>[2x]MTKPLIKPDVDLTDGNFYASRQAREAYRWMRANQPVFRDRNGLAAASTYQAVIDAERQPELFSNAGGIRPDQDALPMMIDMDDPAHLLRRKLVNAGFTRKRVKDKERSIAQLCDTLIDAVCERGECDFVRDLAAPLPMAVIGDM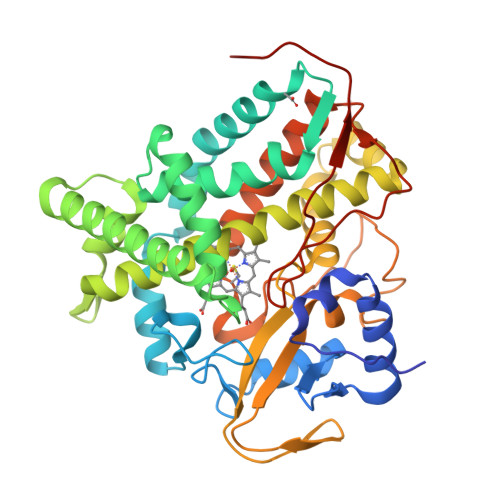LGVLPEQREMFLRWSDDLVTFLSSHVSQEDFQVTIDAFAAYNDFTRATIAARRAEPTDDLVSVLVSSEVDGERLSDDELVMETLLILIGGDETTRHTLSGGSEQLLRNRDQWDLLQSDRELLPGAIEEMLRWTAPVKNMCRMLTADTEFHGTALSEGEKIMLLFESANFDEAVFTDPEKFDIQRNPNSHLAFGFGTHFCMGNQLARLELSLMTARVVQRLPDLRLADQDSRLPLRPANFVSGLESMPVVFTPSRPLSGGSG> MLVEHLRNFSESILESLETAIITLSKDGRITEWNKKAEQLFGLKKENVLGRRLKDLPDFEEIGSVAESVFENKEPVFLNFYKFGERYFNIRFSPFRNAKTQLLEGVIITIDDVTELYKYEEERKRRERLSILGEMTARVAHEIRNPITIIGGFIMRMKKHLDDPETLKKYINIITNELSRLETIVKEILEYSKERQVLEFTEFNLNELIREVYVLFEEKIRKMNIDFCFETDNEDLRVEADRTRIKQVLINLVQNAIEATGENGKIKITSEDMYTKVRVSVWNSGPPIPEELKEKIFSPFFTTKTQGTGLGLSICRKIIEDEHGGKIWTENRENGVVFIFEIPKTPEKR;> MKRILVVDDEPNIR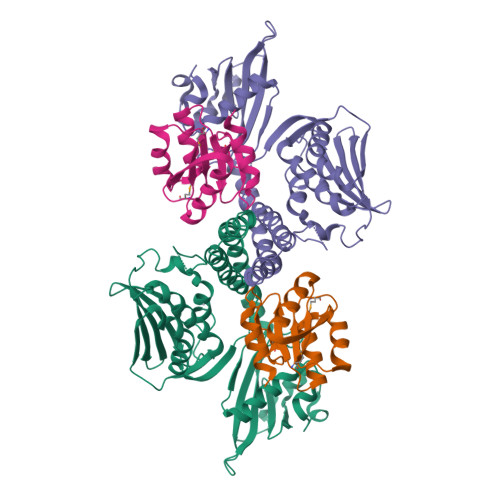ELLKEELQEEGYEIDTAENGEEALKKFFSGNYDLVILDIEMPGISGLEVAGEIRKKKKDAKIILLTAYSHYRSDMSSWAADEYVVKSFNFDELKEKVKKLLS>MGSSHHHHHHSQDPMVLLHKSTHIFPTDFASVSRAFFNRYPNPYSPHVLSIDTISRNVDQEGNLRTTRLLKKSGKLPTWVKPFLRGITETWIIEVSVVNPANSTMKTYTRNLDHTGIMKVEEYTTYQFDSATSSTIADSRVKFSSGFNMGIKSKVEDWSRTKFDENVK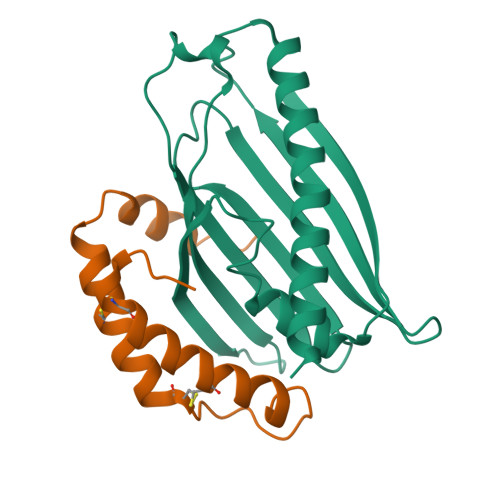KSRMGMAFVIQKLEEARNPQF[2x];>[2x]MGNIMSASFAPECTDLKTKYDSCFNEWYSEKFLKGKSVENECSKQWYAYTTCVNAALVKQGIKPALDEAREEAPFENGGKLKEVDK> MADYKDDDDKSGPDEVDASGRMAVLRQLALLLWKNYTLQKRKVLVTVLELFLPLLFSGILIWLRLKIQSENVPNATIYPGQSIQELPLFFTFPPPGDTWELAYIPSHSDAAKTVTETVRRALVINMRVRGFPSEKDFEDYIRYDNCSSSVLAAVVFEHPFNHSKEPLPLAVKYHLRFSYTRRNYMWTQTGSFFLKETEGWHTTSLFPLFPNPGPREPTSPDGGEPGYIREGFLAVQHAVDRAIMEYHADAATRQLFQRLTVTIKRFPYPPFIADPFLVAIQYQLPLLLLLSFTYTALTIARAVVQEKERRLKEYMRMMGLSSWLHWSAWFLLFFLFLLIAASFMTLLFCVKVKPNVAVLSRSDPSLVLAFLLCFAISTISFSFMVSTFFSKANMAAAFGGFLYFFTYIPYFFVAPRYNWMTLSQKLCSCLLSNVAMAMGAQLIGKFEAKGMGIQWRDLLSPVNVDDDFCFGQVLGMLLLDSVLYGLVTWYMEAVFPGQFGVPQPWYFFIMPSYWCGKPRAVAGKEEEDSDPEKALRNEYFEAEPEDLVAGIKIKHLSKVFRVGNKDRAAVRDLNLNLYEGQITVLLGHNGAGKTTTLSMLTGLFPPTSGRAYISGYEISQDMVQIRKSLGLCPQHDILFDNLTVAEHLYFYAQLKGLSRQKCPEEVKQMLHIIGLEDKWNSRSRFLSGGMRRKLSIGIALIAGSKVLILDEPTSGMDAISRRAIWDLLQRQKSDRTIVLTTHFMDEADLLGDRIAIMAKGELQCCGSSLFLKQKYGAGYHMTLVKEPHCNPEDISQLVHHHVPNATLESSAGAELSFILPRESTHRFEGLFAKLEKKQKELGIASFGASITTMEEVFLRVGKLVDSSMDIQAIQLPALQYQHERRASDWAVDSNLCGAMDPSDGIGALIEEERTAVKLNTGLALHCQQFWAMFLKKAAYSWREWKMVAAQVLVPLTCVTLALLAINYSSELFDDPMLRLTLGEYGRTVVPFSVPGTSQLGQQLSEHLKDALQAEGQEPREVLGDLEEFLIFRASVEGGGFNERCLVAASFRDVGERTVVNALFNNQAYHSPATALAVVDNLLFKLLCGPHASIVVSNFPQPRSALQAAKDQFNEGRKGFDIALNLLFAMAFLASTFSILAVSERAVQAKHVQFVSGVHVASFWLSALLWDLISFLIPSLLLLVVFKAFDVRAFTRDGHMADTLLLLLLYGWAIIPLMYLMNFFFLGAATAYTRLTIFNILSGIATFLMVTIMRIPAVKLEELSKTLDHVFLVLPNHCLGMAVSSFYENYETRRYCTSSEVAAHYCKKYNIQYQENFYAWSAPGVGRFVASMAASGCAYLILLFLIETNLLQRLRGILCALRRRRTLTELYTRMPVLPEDQDVADERTRILAPSPDSLLHTPLIIKELSKVYEQRVPLLAVDRLSLAVQKGECFGLLGF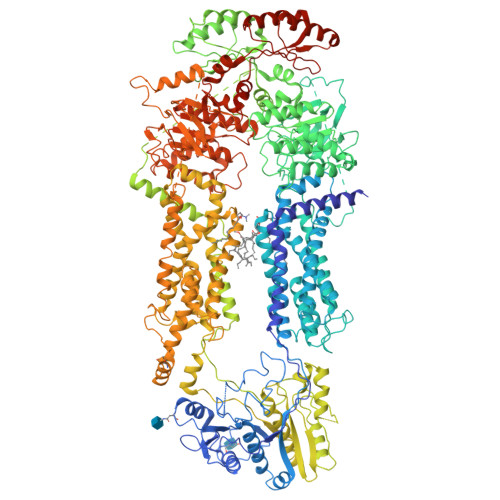NGAGKTTTFKMLTGEESLTSGDAFVGGHRISSDVGKVRQRIGYCPQFDALLDHMTGREMLVMYARLRGIPERHIGACVENTLRGLLLEPHANKLVRTYSGGNKRKLSTGIALIGEPAVIFLDEPSTGMDPVARRLLWDTVARARESGKAIIITSHSMEECEALCTRLAIMVQGQFKCLGSPQHLKSKFGSGYSLRAKVQSEGQQEALEEFKAFVDLTFPGSVLEDEHQGMVHYHLPGRDLSWAKVFGILEKAKEKYGVDDYSVSQISLEQVFLSFAHLQPPTAEEGRLEGSDEVDAVEGSHHHHHHHHHH>GGUACACGACAAUACUAAACCAUCCGCGAGGAUGGGGCGGAAAGCCUAAGGGUCUCCCUGAGACAGCCGGGCUG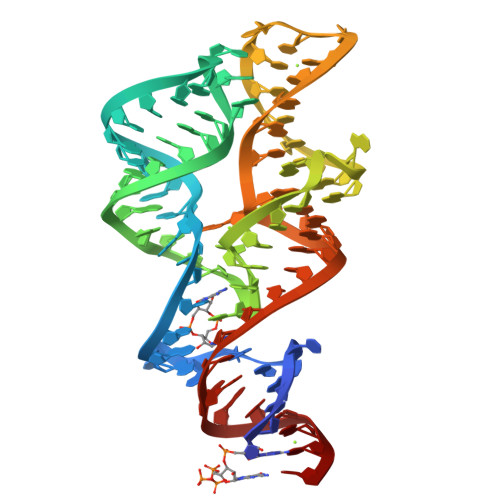CCGAAAUAUC[2x]> MPWEDYVGKTLPVGSRLPPNFKTYDYFDRATGAVVSAKSLDTQTMAKLSNPNQVYSSIKKNIDVTAKFEKASLSGVTVNSSMITSKEVRLAVPVNTTKAQWTEINRAI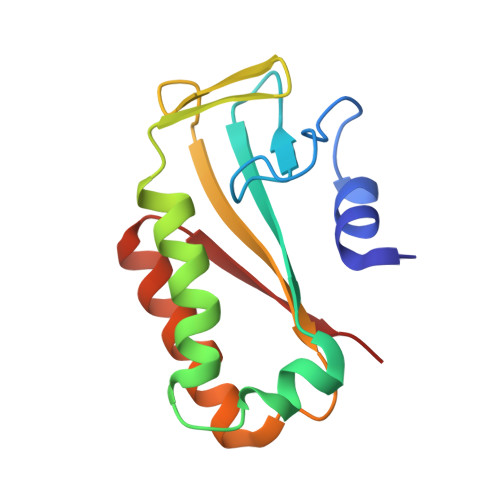EYGKNQGVKVTVTQVK>[2x]MQIKTVTFENNRGERLAARLDLPVDTQPVAYALFAHCFTCSKNLKAVTTISRALTTQGYAVLRFDFTGLGESEGDFSETTFATNFEDLRAACRFLSAQYEPPALLIGHSLGGAAVLAVAGEFPE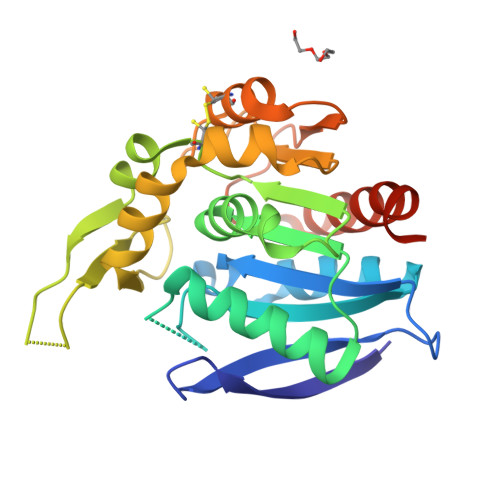VKAVATIGAPCDPAHVRHLLRPALDTIKTVGEAVVDLGGRPFRIKKQFLEELERVNLEDQVRTMRRPLLLFHSPTDQIVGIENAACLFQAARHPKSFVSLDQADHLLSNSDDAAFVGEVLGAWARRYVGRRLGHHHHHH>EDVEIKPRGYQLRLVDHLTKSNGIVYLPTGSGKTFVAILVLKRFSQDFDKPIESGGKRALFMCNTVELARQQAMAVRRCTNFKVGFYVGEQGVDDWTRGMWSDEIKKNQVLVGTAQVFLDMVTQTYVALSSLSVVIIDECHHGTGHHPFREFMRLFTIANQTKLPRVVGLTGVLIKGNEITNVATKLKELEITYRGNIITVSDTKEMENVMLYATKPTEVMVSFPHQEQVLTVTRLISAEIEKFYVSLDLMNIGVQPIRRSKSLQCLRDPSKKSFVKQLFNDFLYQMKEYGIYAASIAIISLIVEFDIKRRQAETLSVKLMHRTALTLCEKIRHLLVQKLQDMTYDDDDDNVNTEEVIMNFSTPKVQRFLMSLKVSFADKDPKDICCLVFVERRYTCKCIYGLLLNYIQSTPELRNVLTPQFMVGRNNISPDFESVLERKWQKSAIQQFRDGNANLMICSSVLEEGIDVQACNHVFILDPVKTFNMYVQSKGRARTTEAKFVLFTADKEREKTIQQIYQYRKAHNDIAEYLKDRVLEKTEPELYEIKGHFQDDIDPFTNENGAVLLPNNALAILHRYCQTIPTDAFGFVIPWFHVLQEDERDRIFGVSAKGKHVISINMPVNCMLRDTIYSDPMDNVKTAKISAAFKACKVLYSLGELNERFVPKTLKERVASIADVHFEHWNKYGDSVTATVNKADKSKDRTYKTECPLEFYDALPRVGEICYAYEIFLEPQFESCEYTEHMYLNLQTPRNYAILLRNKLPRLAEMPLFSNQGKLHVRVANAPLEVIIQNSEQLELLHQFHGMVFRDILKIWHPFFVLDRRSKENSYLVVPLILGAGEQKCFDWELMTNFRRLPQSHGSNVQQREQQPAPRPEDFEGKIVTQWYANYDKPMLVTKVHRELTPLSYMEKNQQDKTYYEFTMSKYGNRIGDVVHKDKFMIEVRDLTEQLTFYVHNRGKFNAKSKAKMKVILIPELCFNFNFPGDLWLKLIFLPSILNRMYFLLHAEALRKRFNTYLNLHLLPFNGTDYMPRPLEIDYSLKRNVDPLGNVIPTEDIEEPKSLLEPMPTKSIEASVANLEITEFENPWQKYMEPVDLSRNLLSTYPVELDYYYHFSVGNVCEMNEMDFEDKEYWAKNQFHMPTGNIYGNRTPAKTNANVPALMPSKPTVRGKVKPLLILQKTVSKEHITPAEQGEFLAAITASSAADVFDMERLEILGNSFLKLSATLYLASKYSDWNEGTLTEVKSKLVSNRNLLFCLIDADIPKTLNTIQFTPRYTWLPPGISLPHNVLALWRENPEFAKIIGPHNLRDLALGDEESLVKGNCSDINYNRFVEGCRANGQSFYAGADFSSEVNFCVGLVTIPNKVIADTLEALLGVIVKNYGLQHAFKMLEYFKICRADIDKPLTQLLNLELGGKKMRANVNTTEIDGFLINHYYLEKNLGYTFKDRRYLLQALTHPSYPTNRITGSYQELEFIGNAILDFLISAYIFENNTKMNPGALTDLRSALVNNTTLACICVRHRLHFFILAENAKLSEIISKFVNFQESQGHRVTNYVRILLEEADVQPTPLDLDDELDMTELPHANKCISQEAEKGVPPKGEFNMSTNVDVPKALGDVLEALIAAVYLDCRDLQRTWEVIFNLFEPELQEFTRKVPINHIRQLVEHKHAKPVFSSPIVEGETVMVSCQFTCMEKTIKVYGFGSNKDQAKLSAAKHALQQLSKCDA[2x];>[2x]MDQENFHGSSLPQQLQNLHIQPQQASPNPVQTGFAPRRHYNNLVGLGNGNAVSGSPVKGAPLGQRHVKLKKEKISAQVAQLSQPGQLQLSDVGDPALAGGSGLQGGVGLMGVILPSDEALKFVSETDANGLAMKTPVSILQELLSRRGITPGYELVQIEGAIHEPTFRFRVSFKDKDTPFTAMGAGRSKKEAKHAAARALIDKLIGAQLPESPSSSAGPSVTGLTVAGSGGDGNANATGGGDASDKTVGNPIGWLQEMCMQRRWPPPSYETETEVGLPHERLFTIACSILNYREMGKGKSKKIAKRLAAHRMWMRLQETPID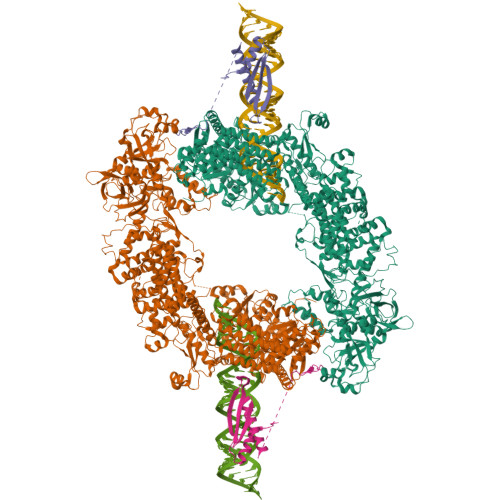SGKISDSICGELEGEVSIIQDIDRYEQVSKDFEFIKI>MAHHHHHHMSVKVFDTKEVQDLLKAASNAGTNGANGTQAGNARTQQIVHRLLGDLFKAIDDLDITPDEVWAGVNYLNKLGQDGEAALLAAGLGLEKYLDIRMDAEDEAIGLDGG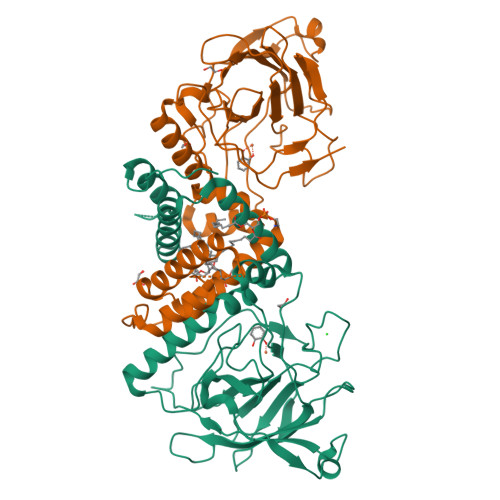TPRTIEGPLYVAGAPVRDGVAKIDLDADEGAGPLVIHGTVTGLDGKPVAGALVECWHANSHGFYSHFDPTGKQSDFNLRGAVKTGADGKYEFRTLMPVGYGCPPQGATQQLLDRLGRHGNRPAHVHFFVTSDGHRKLTTQFNIEGDPLIWDDFAYATREELIPPVTAKAGGAALGLKADAYQDIEFNFVLTPRVEGKDNQIVERLRASATA[2x]> AVSLDRTRAVFDGSEKSMTLDISNDNKQLPYLAQAWIENENQEKIITGPVIATPPVQRLEPGAKSMVRLSTTPDISKLPQDRESLFYFNLREIPPRSEKANVLQIALQTKIKLFYRPAAIKTRPNEVWQDQLILNKVSGGYRIENPTPYYVTVIGLGGSEKQAEEGEFETVMLSPRSEQTVKSANYNTPYLSYINDYGGRPVLSFICNGSRCSVKKEK;> SDVAFRGNLLDRPCHVSGDSLNKHVVFKTRASRDFWYPPGRSPTESFVIRLENCHATAVGKIVTLTFKGTEEAALPGHLK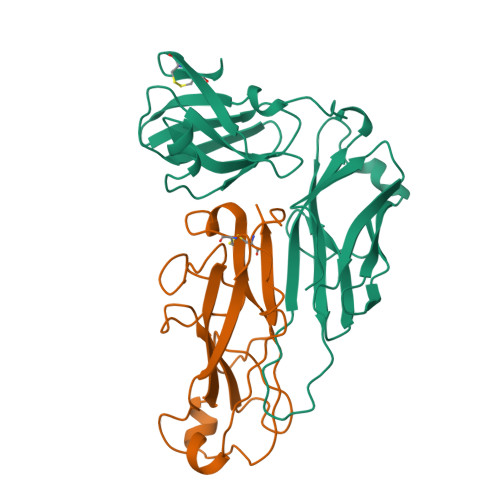VTGVNAGRLGIALLDTDGSSLLKPGTSHNKGQGEKVTGNSLELPFGAYVVATPEALRTKSVVPGDYEATATFELTYR Unlike most other members of enveloped viruses that utilize one or a limited number of viral proteins for entry, poxvirus encodes four (A26, A27, D8 and H3, protein names refer to VACV) and another eleven proteins (A16, A21, A28, F9, G3, G9, H2, J5, L1, L5 and O3, protein names refer to VACV) to mediate attachment and membrane fusion, respectively. For the eleven fusion associated proteins, they are proposed to assemble into a large machinery, called the entry-fusion complex (EFC). In this study, we carried out structural characterization on VACV G3 and L5 proteins. These two EFC-component proteins, have been previously shown to interact with each other to form a stable sub-complex, and show highly conserved amino-acid sequences among orthopoxviruses.

Eventually, we solved the sub-complex structures at 1.8-Å (for P21 space group) and 1.5-Å (for P31 space group) resolutions using the single-wavelength anomalous dispersion method, respectively. The Rwork/Rfree values were refined to 0.202/0.221 (for P21 space group) and 0.190/0.206 (for P31 space group), respectively. Because protein terminus residues are much better traced in the electron density map for the structure with the P21 space group than the structure with the P31 space group, description of the structural elements below is based on the P21 structure unless otherwise specified. The complex structure, within the crystallographic asymmetric unit, contains G3 (amino acids A40-K111) and L5 (residues K60-R128) in single 1:1 binding mode. As can be viewed from the overall structure, G3 and L5, with good shape complementarity, are stacked together to form a globular fold. G3 consists of four anti-parallel β-strands (β1-β4) and two α-helices (α1-α2), assembling into a compact structure (Figure 1(F,G)). Helix-α1 intersperses the β-sheet on the lateral side. L5 is composed of three anti-parallel β-strands (β1’-β3’), two α-helices (α1’-α2’) and one 310 helix (η1’) (Figure 1(F,G)). One conserved disulfide bond is observed between C75 in β1’-strand and C107 in α1’-helix to stabilize the structure. On the whole, large surface areas are buried in the sub-complex, which are calculated to be ∼1606 Å2 for G3 and ∼1553 Å2 for L5, respectively. The extended binding interface can be further subdivided into three binding patches (Patch1, 2 and 3) based on the G3 elements involved in L5-engagement. In comparison to the other two patches, the third patch therefore shows the best overall structural complementarity, the largest number of participating amino acids, and the most diverse types of inter-chain contacts (van der Waals, hydrophobic interactions and hydrogen bonds). Taken together, a total of 15 residues in G3 and 18 amino acids in L5 are positioned along the binding interface, providing extended inter-molecule interactions for sub-complex formation (Figure 1(M,N)).

> GPYYPTNKLQAAVMETDRENAIIRQRNDEIPTRTLDTAIFTDASTVASAQIHLYYNSNIGKIIMSLNGKKHTFNLYDDNDIRTLLPILLLSK;> GPNMFFMPKRKIPDPIDRLRRANLACEDDKLMIYGLPWMTTQTSALSINSKPIVYKDCAKLLRSINGSQPVSLNDVLRR> ADPRGHNFCAEGPKCGENSECKNWNTKATCECKSGYISVQGDSAYCEDIDECAAKMHYCHANTVCVNLPGLYRCDCVPGYIRVDDFSCTEHD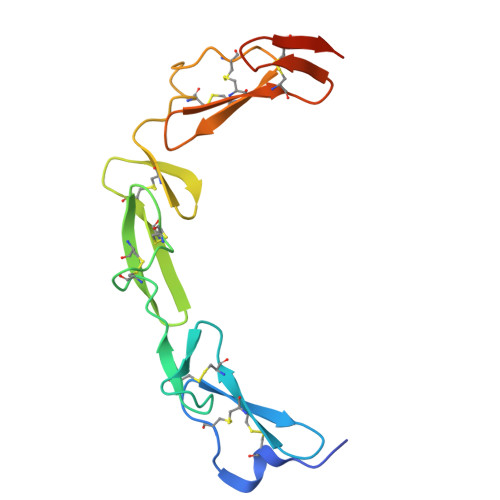ECGSGQHNCDENAICTNTVQGHSCTCKPGYVGNGTICRAEFHHHHHH> TFRYRGPSPKGDQPKAIAGLVEALRDGERFVTLLGATGTGKTVTMAKVIEALGRPALVLAPNKILAAQLAAEFRELFPENAVEYFISYYDYYQPEAYVPGKDLYIEKDASINPEIERLRHSTTRSLLTRRDVIVVASVSAIYGLGDPREYRARNLVVERGKPYPREVLLERLLELGYQRNDIDLSPGRFRAKGEVLEIFPAYETEPIRVELFGDEVERISQVHPVTGERLRELPGFVLFPATHYLSPEGLEEILKEIEKELWERVRYFEERGEVLYAQRLKERTLYDLEMLRVMGTCPGVENYARYFTGKAPGEPPYTLLDYFPEDFLVFLDESHVTVPQLQGMYRGDYARKKTLVDYGFRLPSALDNRPLRFEEFLERVSQVVFVSATPGPFELAHSGRVVEQIIRPTGLLDPLVRVKPTENQILDLMEGIRERAARGERTLVTVLTVRMAEELTSFLVEHGIRARYLHHELDAFKRQALIRDLRLGHYDCLVGINLLREGLDIPEVSLVAILDADKEGFLRSERSLIQTIGRAARNARGEVWLYADRVSEAMQRAIEETNRRRALQEAYNLEHGITPETVRKEVRAVIRPEGYEEAPLEADLSGE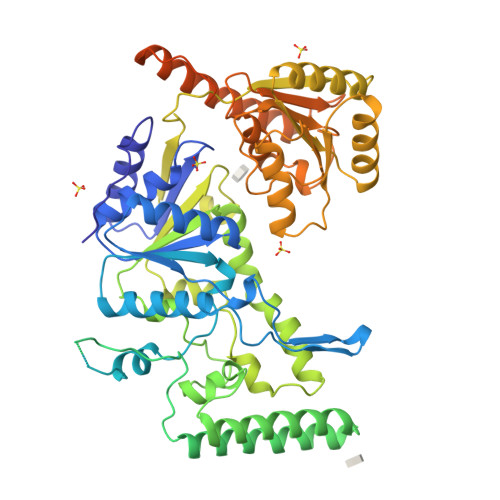DLRERIAELELAMWQAAEALDFERAARLRDEIRALEARLQGVRAPEPVPGGRKRKRR>[2x]NAQFLHTQVGRGLLGAVVNPLGEVTDKFAVTDNSEILYRPVDNAPPLYSERAAIEKPFLTGIKVIDSLLTCGEGQRMGIFASAGCGKT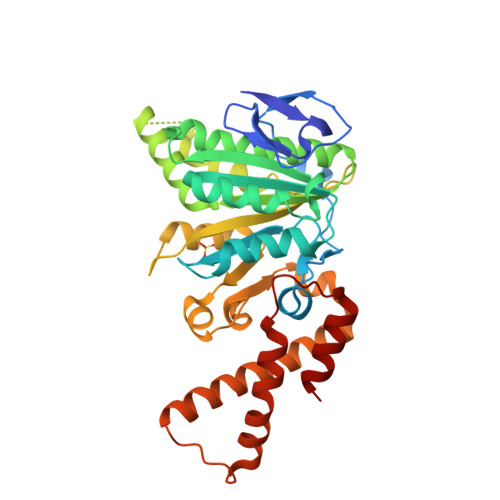FLMNMLIEHSGADIYVIGLIGARGREVTETVDYLKNSEKKSRCVLVYATSDYSSVDRCNAAYIATAIAEFFRTEGHKVALFIDSLTRYARALRDVALAAGESPARRGYPVSVFDSLPRLLERPGKLKAGGSITAFYTVLLEDDDFADPLAEEVRSILDGHIYLSRNLAQKGQFPAIDSLKSISRVFTQVVDEKHRIMAAAFRELLSEIEELRTIIDFGEYKPGENASQDKIYNKISVVESFLKQDYRLGFTYEQTMELIGETIR>MAVKKIAIFGATGQTGLTTLAQAVQAGYEVTVLVRDSSRLPSEGPRPAHVVVGDVLQAADVDKTVAGQDAVIVLLGTRNDLSPTTVMSEGARNIVAAMKAHGVDKVVACTSAFLLWDPTKVPPRLQAVTD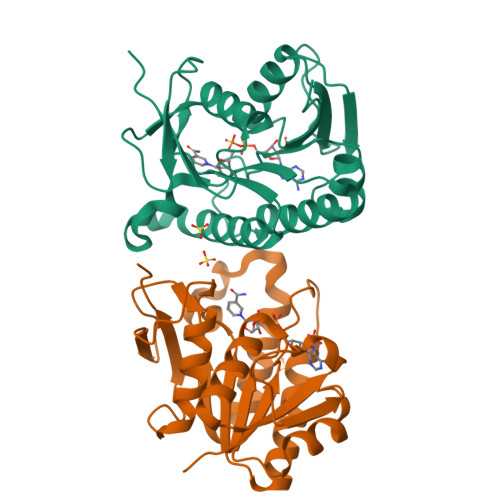DHIRMHKVLRESGLKYVAVMPPHIGDQPLTGAYTVTLDGRGPSRVISKHDLGHFMLRCLTTDEYDGHSTYPSHQYQ[2x]N-[(S)-[(2R)-2-(benzoylamino)-2-carboxyethoxy](hydroxy)phosphoryl]-L-glutamic acid | C15 H19 N2 O10 P | 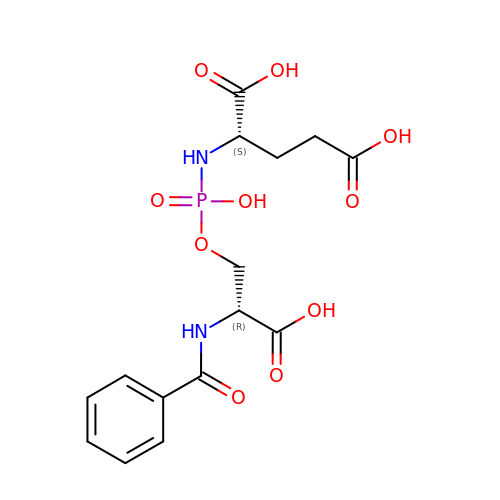FMKMCQXFKJRGIQ-WDEREUQCSA-N4-oxo-N-(4-sulfamoylphenethyl)-1,3,4,6,7,11b-hexahydro-2H-pyrazino[2,1-a]isoquinoline-2-carbothioamide 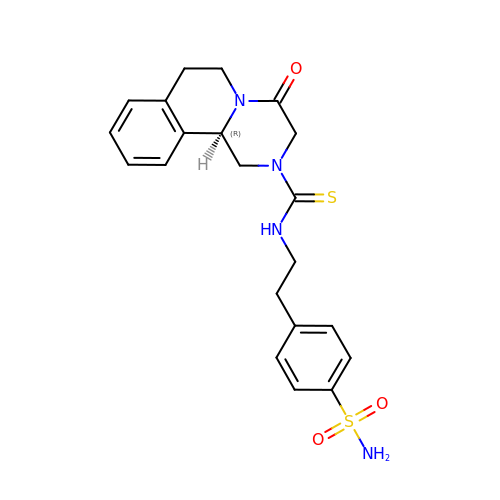| C21 H24 N4 O3 S2 | WAXCPJVEJJWBNS-IBGZPJMESA-N>HLNVLAKALYDNVAESPDELSFRKGDIMTVLEQDTQGLDGWWLCSLH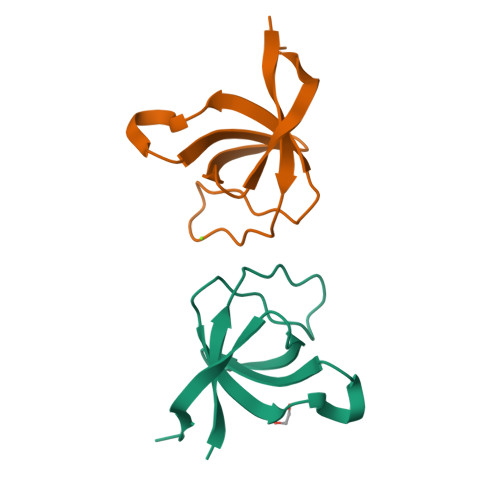GRQGIVPGNRLKILVGMYDKKP[2x]>[6x]AANRELQASLNLLQEDQNAGRQVQMNMLPVTPWSIEGLEFSHRIIPSLYLSGDFVDYFRVDERRVAFYLADVSGHGASSAFVTVLLKFMTTRLLYESRRNGTLPEFKPSEVLAHINRGLINTKLGKHVTMLGGVIDLEKNSLTYSIGGHLPLPVLFVEGQAGYLEGRGLPVGLFDDATYDDRVMELPPSFSLSLFSDGILDVLPGATLKEKEASLPEQVAAAGGTLDGLRQVFGLA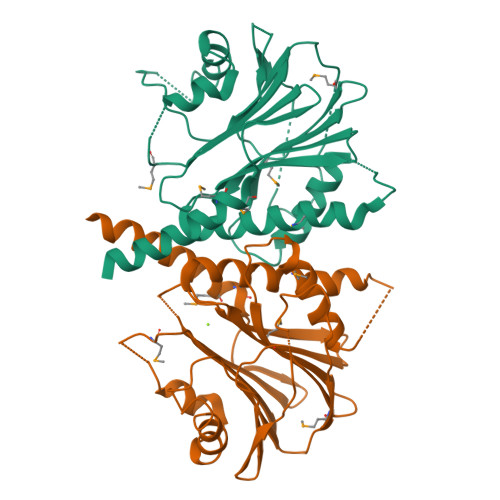NLAEMPDDIALLVLSRNLA>SMQVQLPKKFENPKNVRIALVREVGEGSFFERYLAGAQSMARELGVTLLEATAHGDMARMVTMIENFITQRVDAIIIDHGRPDPLMPKIKEALDRGIRVVTFDLVVDDNRVPEIEQDDLLIGYLISKQLAVDFAGNANVIYVNVGGFAPLDKRDKMWQIIKWRFPGIKEVAKIGAVTGSTAADTQTRMEAAMKEKPEANAVLAMWDEFAKGAVRAIMQAGKSDQFKVYSVDVTTEDIQMMIQQNSPWVATVGTDSYAVGRLAVRAAAALVGGEKLPKYLLVEP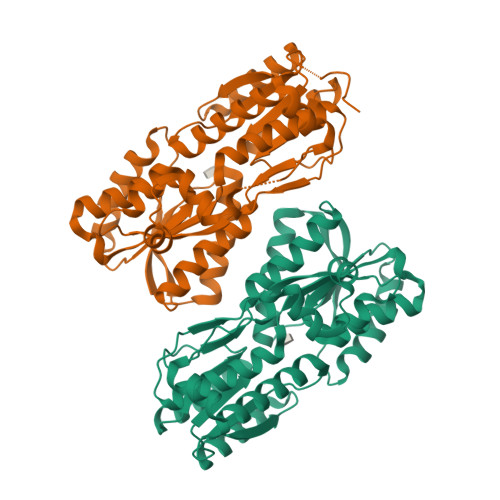QLITRQFLVDNNITNMDELVKALPALGESNLVWPEWLKALTEKNKK[4x]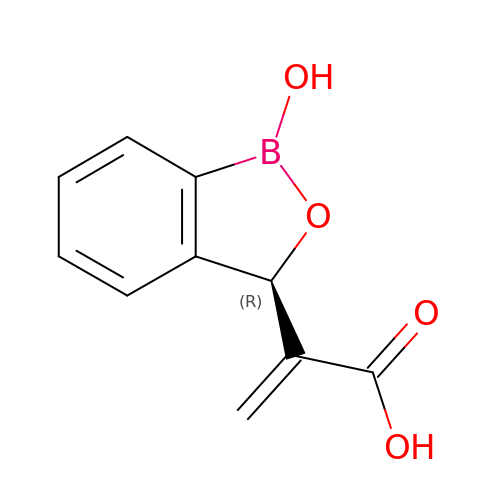2-[(3R)-1-oxidanyl-3H-2,1-benzoxaborol-3-yl]prop-2-enoic acid | C10 H9 B O4 | BRBGRVSFRVLGNY-VIFPVBQESA-N4-(hydroxymethyl)-1-beta-L-mannopyranosyl-1H-1,2,3-triazole | C9 H15 N3 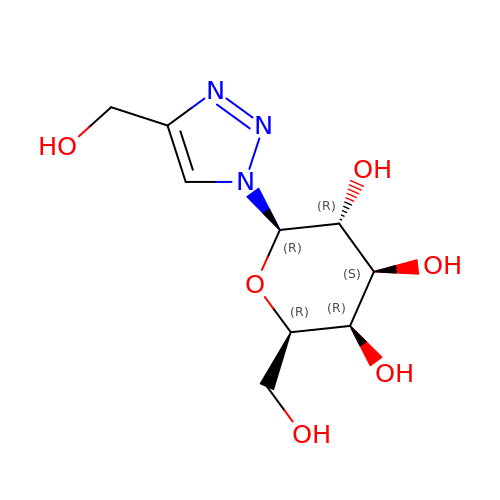O6 | BHGZOVXPACYZLI-WMOCKQOXSA-N>MKHHHHHHHHGGLVPRGSHGGSEFQVRSFEEIKRSGEIRIGTEGAFPPFNYFDERNQLTGFEVDLGNAIAERLGLKPRWIAQSFDTLLIQLNQGRFDFVIASHGITEERARAVDFTNPHYCTGGVIVSRKGGPRTAKDLQGKVVGVQVGTTYMEAAQKIPGIKEVRTYQRDPDALQDLLAGRIDTWITDRFVAKEAIKERKLENTLQVGELVFQERVAMAVAKGNKSLLDALNRALAE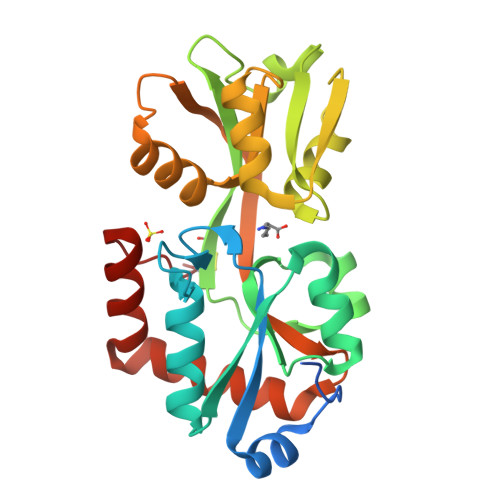LMQDGTYARISQKWFGEDVRCK[2x]3'-O-ACETYLTHYMIDINE-5'-DIPHOSPHATE | C12 H18 N2 O12 P2 | 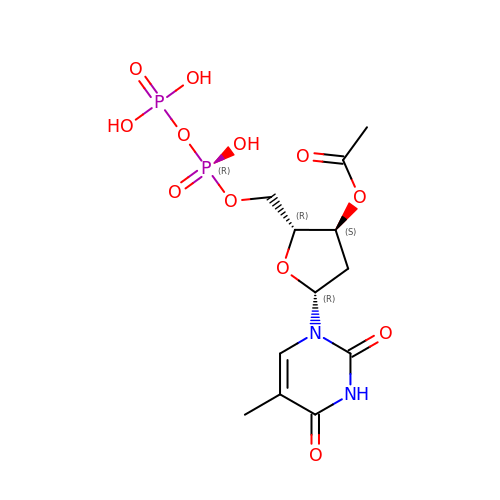UWSIAAWKEICIJY-IVZWLZJFSA-N>ADPHHHHHHHHTPQPCQAPQQWEGRQVLYQQSSGHNNRALVSYDGLNQRVRVLDERKALIPCKRLFEYILLYKEGVMFQIEQATKQCAKIPLVESWDPLDIPQNSTFEDQYSIGGPQEQILVQEWSDRRTARSYETWIGVYTAK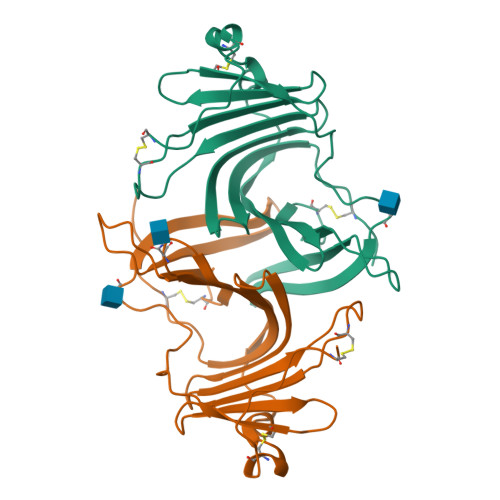DCYPVQETFIRNYTVVMSTRFFDVQLGIKDPSVFTPPSTCQAAQPEKMSDGCSL[4x]> PPKELVNEWSLKIRKEMRVVDRQIRDIQREEEKVKRSVKDAAKKGQKDVCIVLAKEMIRSRKAVSKLYASKAHMNSVLMGMKNQLAVLRVAGSLQKSTEVMKAMQSLVKIPEIQATMRELSKEMMKAGIIEEMLEDTFESMDDQEEMEEEAEMEIDRIL;> RKTPEELLRQNQRALNRAMRELDRERQKLETQEKKIIADIKKMAKQGQMDAVRIMA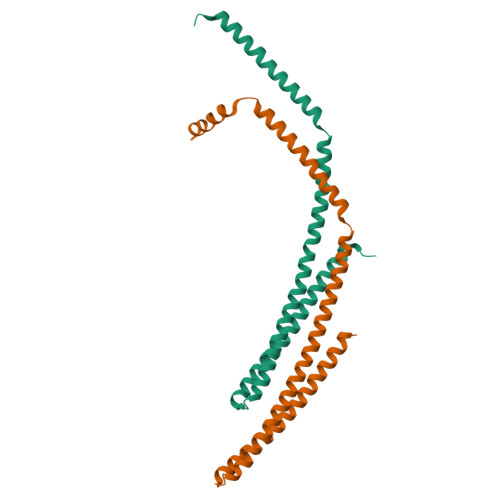KDLVRTRRYVRKFVLMRANIQAVSLKIQTLKSNNSMAQAMKGVTKAMGTMNRQLKLPQIQKIMMEFERQAEIMDMKEEMMNDAIDDAMGDE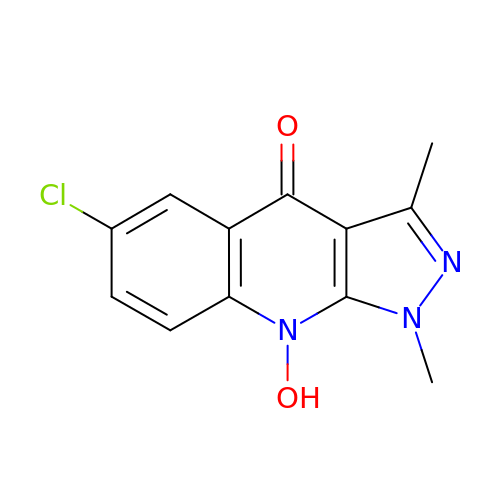6-CHLORO-9-HYDROXY-1,3-DIMETHYL-1,9-DIHYDRO-4H-PYRAZOLO[3,4-B]QUINOLIN-4-ONE | C12 H10 Cl N3 O2 | AYKGPCNWPACUQV-UHFFFAOYSA-N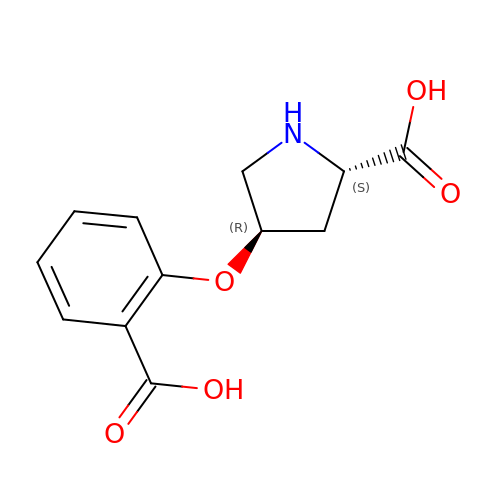(2~{S},4~{R})-4-(2-carboxyphenoxy)pyrrolidine-2-carboxylic acid | C12 H13 N O5 | XHABYXGKUZQAIW-APPZFPTMSA-N> MASMTGGQQMGAPITAYAQQTRGLLGCIITSLTGRDKNQVEGEVQIVSTATQTFLATCING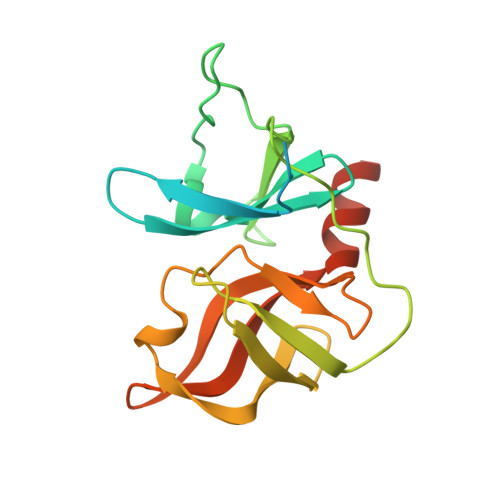VCWTVYHGAGTRTIASPKGPVIQMYTNVDQDLVGWPAPQGSRSLTPCTCGSSDLYLVTRHADVIPVRRRGDSRGSLLSPRPISYLKGSSGGPLLCPAGHAVGLFRAAVCTRGVAKAVDFIPVENLETTMRSGSHHHHHH> GP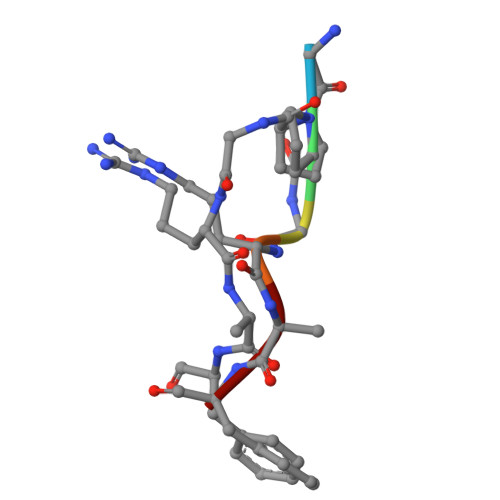GRAF> DPSVTHVLHQLCDILANNYAFSERIPTLLQHLPNLDYSTVISEEDIAAKLNYELQSLT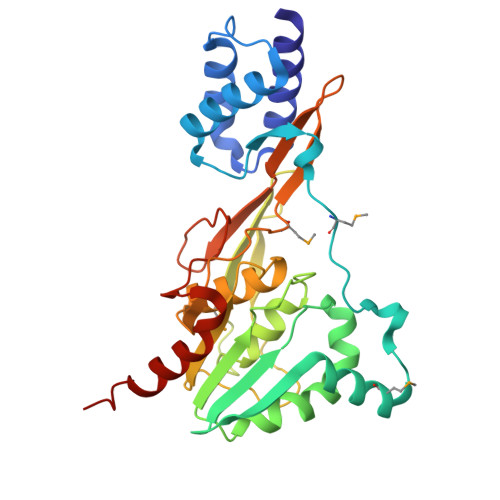EDPRLVLKSKTDTLVMPGDSIQAENIPEDEAMLQALVNTVFKVSILPGNIGYLRFDQFADVSVIAKLAPFIVNTVWEPITITENLIIDLRYNVGGSSTAVPLLLSYFLDPETKIHLFTLHNRQQNSTDEVYSHPKVLGKPYGSKKGVYVLTSHQTATAAEEFAYLMQSLSRATIIGEITSGNLMHSKVFPFGDTQLSVTVPIINFIDSNGDYWLGGGVVPDAIVLADEALDKAKEIIAFHPPLA> MSLSSWRQFQLFENIPIRDPNFGGDSLLYSDPTLCAATIVDPQTLIIAVNSNIIKVVKLNQSQVIHEFQSFPHDFQITFLKVINGEFLVALAESIGKPSLIRVYKLEKLPNREQLYHSQVELKNGNNTYPISVVSISNDLSCIVVGFINGKIILIRGDISRDRGSQQRIIYEDPSKEPITALFLNNDATACFAATTSRILLFNTTGRNRGRPSLVLNSKNGLDLNCGSFNPATNEFICCLSNFIEFFSSSGKKHQFAFDLSLRKRIFCVDKDHILIVTEETGVPTTSISVNELSPTIINRIFIIDAKNKIISLNFVVSSAIIDIFSTSQSGKNITYLLTSEGVMHRITPKSLENQINIIIQKELYPFALQLAKQHSLSPLDVQEIHKKYGDYLFKKGLRKEATDQYIQCLDVVETSEIISKFGVKEVPDPESMRNLADYLWSLIKNSISQRDHVTLLLIVLIKLKDVEGIDTFIQHFDRKGIWNEGVVMDDMDDVTFFYSDNDFFDLDLILELMKESDFKRLSYRLAKKYSKDSLIIVDILLNLLHNPVKAIKYIKSLPIDETLRCLVTYSKKLLEESPNETNALLIEVFTGKFKPSTFEVDLDRRDTTGDFSENIRTVFYSYKTFFNYMNSNGTSDAMSESSEASHEHEEPTYHPPKPSIVFSSFVTKPFEFVVFLEACLACYQQYEGFDEDRQVILTTLYDLYLNLAQNDVPERIDDWRSRATGVLRESNKLVYSAASNNTSKRVDNSIMLLISHMDQSSASAKDKTKIDIASFANDNPEMDLLSTFRAMTLNEEPSTCLKFLEKYGTEEPKLLQVALSYFVSNKLIFKEMGGNEVLKEKVLRPIIEGERMPLLDIIKALSRTNVAHFGLIQDIIIDHVKTEDTEIKRNEKLIESYDKELKEKNKKLKNTINSDQPLHVPLKNQTCFMCRLTLDIPVVFFKCGHIYHQHCLNEEEDTLESERKLFKCPKCLVDLETSNKLFEAQHEVVEKNDLLNFALNSEEGSRDRFKVITEFLGRGAISYSDITI;> MKNPSFDWERLKDVFYRSRAIGELKWPTQYEEFKCALSLTVIAVEIQDFIQVYNYFGQLLGKINLQRIHEDIIKFEFDKDEKLILVTKSSIKIVKGWSPLTIESVPLQDPTI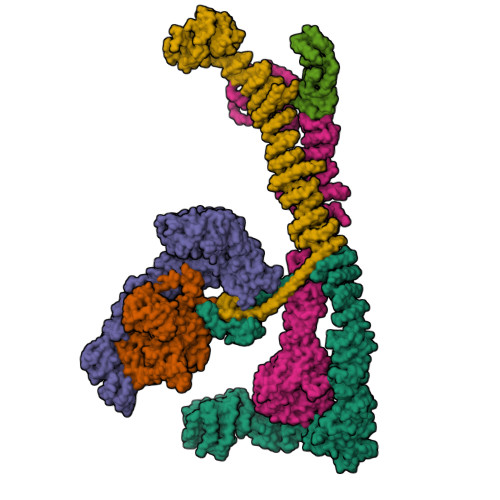DTIWDYHNGIMLLAKSRDIYKLNGNEWELLYENKDKKYNLLTKNHWSCNDDSIILLDVDHVYQVSTSNGALLKLITDSSWHKVTISSRGFICLYNMKDNKLQIFRDPARILMEHNLDSTPDDICWCGNDTVACSFEDEIKLYGPDGLYVTFWYPFTVTNLRAEVDGLKVITTEKIYFLSRVQPQTSNIFRIGSTEPGAMLVDSFSLLEDHAPKAIEILKNFVLEKGVLDCIAAAIDEFEPKLQKMLLNAASYGKASLQYKSFDASIFVNACNTIKLLNCFRSFGIFLTVEEYRCISLKGVIDRLLKYHRYYECIQICKLANERFLLGYVFTEWAKDKIKGSPDMEDDELLDKIKSRLSVIDMTDTLQMVAVAKVAYLEGRFQLSRNLALLEKNEEARIEQLYNLDDDSIALKECIKVQNYSLTISLLIALSKKLTNSQLTKLLIIDMFNNPLYLYYMRMDKAYLYDFYRQTDRFIDLAHVLLQQGKEQQSLHSFLPQIKDLYSQVQNSEVVNNTIEQLQRQEKLWIYQESLGKRFAISFTNMTLDQTLSKLIETGQDKQVKEIVKKFKISEKKLYHLKCKTLVEAKKFDELLQFAQSRKSPIGYMPFYTYLKSRGHMDKASPYVNMIPGLSYQEKKKLYVECRGFRDAIQLAGKEKDIPGLKEIYNIIPPNEPELKALANETMSRI;> MIKTRIEEVQLQFLTGNTELTHLKVSNDQLIVTTQRTIYRINLQDPAIVNHFDCPLSKELETIMNVHVSPMGSVILIRTNFGRYMLLKDGEFTQLNKIKNLDLSSLHWINETTFLMGIKKTPKLYRVELTGKDITTKLWYENKKLSGGIDGIAYWEGSLLLTIKDNILYWRDVTNMKFPLVLPDESEQFERLKHHAIKKFDSYNGLFAWVTSNGIVFGDLKEKQMEKDPASNNFGKFLSSSKVLLNFELPDYQNDKDHLIKDIVLTAFHILLLRKNTVTMVSQLNNDVVFHETIPRHQLTGSNTDSNEKFLGLVRDSVKETFWCFSNINVFEIIIENEPNSVWNLLVRDNKFDKALSLKGLTVREIESVKLSKAMYLFHTAKDFHSAAQTLGSMKDLSHFGEIALNFLQIKDYNDLNVILIKQLDNVPWKSTQVVLSSWIIWNFMKQLNDIELKINTTKPASTDEDNLLNWNLNLKEKSNELTKFLESHLEKLDNETVYQIMSKQNRQNELLIFASLINDMKFLLSFWIDQGNWYESLKILLTINNHDLVYKYSLILLLNSPEATVSTWMKIKDLDPNKLIPTILKFFTNWQNNSKLITNISEYPENYSLTYLKWCVREVPKMCNPIVYNSILYMMITDPRNDMILENDIIKFMKSNENKYDLNFQLRLSLKFKKTKTSIFLLTRLNLFEDAIDLALKNNLIDDCKVIVNDEILIEDYKLRKRLWLKIAKHLLLSMKDIDIKQLIRTILNDSNEILTIKDLLPFFNEYTTIANLKEELIKFLENHNMKMNEISEDIINSKNLKVEINTEISKFNEIYRILEPGKSCDECGKFLQIKKFIVFPCGHCFHWNCIIRVILNSNDYNLRQKTENFLKAKSKHNLNDLENIIVEKCGLCSDININKIDQPISIDETELAKWNE;> MNRFWNTKKFSLTNADGLCATLNEISQNDEVLVVQPSVLPVLNSLLTFQDLTQSTPVRKITLLDDQLSDDLPSALGSVPQMDLIFLIDVRTSLRLPPQLLDAAQKHNLSSLHIIYCRWKPSFQNTLEDTEQWQKDGFDLNSKKTHFPNVIESQLKELSNEYTLYPWDLLPFPQIDENVLLTHSLYNMENVNMYYPNLRSLQSATESILVDDMVNSLQSLIFETNSIITNVVSIGNLSKRCSHLLKKRIDEHQTENDLFIKGTLYGERTNCGLEMDLIILERNTDPITPLLTQLTYAGILDDLYEFNSGIKIKEKDMNFNYKEDKIWNDLKFLNFGSIGPQLNKLAKELQTQYDTRHKAESVHEIKEFVDSLGSLQQRQAFLKNHTTLSSDVLKVVETEEYGSFNKILELELEILMGNTLNNDIEDIILELQYQYEVDQKKILRLICLLSLCKNSLREKDYEYLRTFMIDSWGIEKCFQLESLAELGFFTSKTGKTDLHITTSKSTRLQKEYRYISQWFNTVPIEDEHAADKITNENDDFSEATFAYSGVVPLTMRLVQMLYDRSILFHNYSSQQPFILSREPRVSQTEDLIEQLYGDSHAIEESIWVPGTITKKINASIKSNNRRSIDGSNGTFHAAEDIALVVFLGGVTMGEIAIMKHLQKILGKKGINKRFIIIADGLINGTRIMNSIS;> MVKKKTNNDKGKEVKENEGKLDIDSESSPHERENDKKKTEDDSLRATESEETNTHNANPNETVRADKFSQEESRPIEDSPHTDKNTAQESCQPSSAEDNVINTDITSLNEKTSTNDEQEKGLPLKISEGPFTISTLLDNVPSDLIYTCCEAYENHIFLGTTTGDLLHYFELERGNYMLVSQTKFDAESNSKIDKILLLPKVEGALILCDNELVLFILPEFAPRPNTTRLKGISDVVICNFSRSSKAYRIYAFHAEGVRLLKISADSLVLTKAFNFKLIDKACAHEETLMVSKLNSYELINLKSSQVIPLFRISETDEDLEPIITSFNEQSEFLVCSGGGSYDSGAMALVVNHHGDIIKGTIVLKNYPRNVIVEFPYIIAESAFQSVDIYSALPSEKSQLLQSITTSGSDLKISKSDNVFTNTNNSEEFKEKIFNKLRLEPLTHSDNKFRIERERAFVEESYEEKTSLIVYNNLGIHLLVPTPMVLRFTSCEESEIDNIEDQLKKLAKKDLTKFEHIEAKYLMSLLLFLMTLHYDHIEDEVMKKWCDFSDKVDIRILFYMFGWKVYSEIWCFHGLINIVERLKSLKLTNKCENILKMLLMMKNELKKKNKTGLLTNDFDDIMKTIDITLFKLRLEKKETITVDMFERESYDEIIREINLHDDKLPRIELLIEIYKEKGEYLKALNLLREAGDYISLVSFIEENLKKLPEDYIKERIADDLLLTLKQGDENTEECAIKKVLKILDMACINKNDFLNKIPAEETSLKVSFIEQLGVQNSNDSKFLFNYYLAKLREIINQSNIWSILGDFIKEYKDDFAYDKTDITNFIHIKLKHSLQCENFSKYYEKCENLKSENEKDDEFINFTFDEISKIDKEHILTLLFFPNELTNWVSSEELLKIYLSFNDFRSVEKYIGKQNLVAVMKQYLDISSLNYSVELVTNLLQRNFELLDDTDIQLKILETIPSVFPVQTISELLLKVLIKYQEKKEESNLRKCLLKNQISISDELSRNFDSQG;> MEQNGLDHDSRSSIDTTINDTQKTFLEFRSYTQLSEKLASSSSYTAPPLNEDGPKGVASAVSQGSESVVSWTTLTHVYSILGAYGGPTCLYPTATYFLMGTSKGCVLIFNYNEHLQTILVPTLSEDPSIHSIRSPVKSIVICSDGTHVAASYETGNICIWNLNVGYRVKPTSEPTNGMTPTPALPAVLHIDDHVNKEITGLDFFGARHTALIVSDRTGKVSLYNGYRRGFWQLVYNSKKILDVNSSKEKLIRSKLSPLISREKISTNLLSVLTTTHFALILLSPHVSLMFQETVEPSVQNSLVVNSSISWTQNCSRVAYSVNNKISVISISSSDFNVQSASHSPEFAESILSIQWIDQLLLGVLTISHQFLVLHPQHDFKILLRLDFLIHDLMIPPNKYFVISRRSFYLLTNYSFKIGKFVSWSDITLRHILKGDYLGALEFIESLLQPYCPLANLLKLDNNTEERTKQLMEPFYNLSLAALRFLIKKDNADYNRVYQLLMVVVRVLQQSSKKLDSIPSLDVFLEQGLEFFELKDNAVYFEVVANIVAQGSVTSISPVLFRSIIDYYAKEENLKVIEDLIIMLNPTTLDVDLAVKLCQKYNLFDLLIYIWNKIFDDYQTPVVDLIYRISNQSEKCVIFNGPQVPPETTIFDYVTYILTGRQYPQNLSISPSDKCSKIQRELSAFIFSGFSIKWPSNSNHKLYICENPEEEPAFPYFHLLLKSNPSRFLAMLNEVFEASLFNDDNDMVASVGEAELVSRQYVIDLLLDAMKDTGNSDNIRVLVAIFIATSISKYPQFIKVSNQALDCVVNTICSSRVQGIYEISQIALESLLPYYHSRTTENFILELKEKNFNKVLFHIYKSENKYASALSLILETKDIEKEYNTDIVSITDYILKKCPPGSLECGKVTEVIETNFDLLLSRIGIEKCVTIFSDFDYNLHQEILEVKNEETQQKYLDKLFSTPNINNKVDKRLRNLHIELNCKYKSKREMILWLNGTVLSNAESLQILDLLNQDSNFEAAAIIHERLESFNLAVRDLLSFIEQCLNEGKTNISTLLESLRRAFDDCNSAGTEKKSCWILLITFLITLYGKYPSHDERKDLCNKLLQEAFLGLVRSKSSSQKDSGGEFWEIMSSVLEHQDVILMKVQDLKQLLLNVFNTYKLERSLSELIQKIIEDSSQDLVQQYRKFLSEGWSIHTDDCEICGKKIWGAGLDPLLFLAWENVQRHQDMISVDLKTPLVIFKCHHGFHQTCLENLAQKPDEYSCLICQTESNPKIVDYKDDDDKDYKDDDDKDYKDDDDK N-{[(1R)-1-carboxy-2-(methylsulfanyl)ethyl]carbamoyl}-L-glutamic 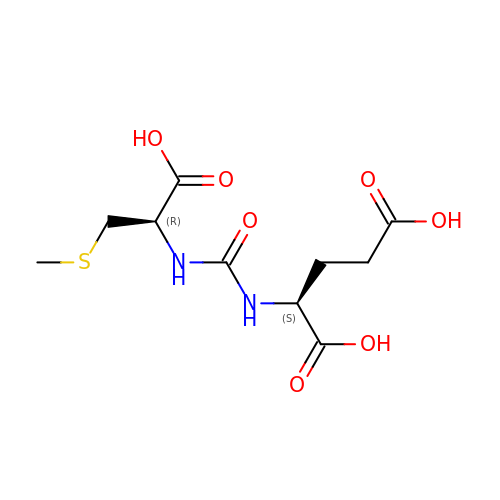acid | C10 H16 N2 O7 S | AUSWZMPQDDVDBG-WDSKDSINSA-N Histones are conserved DNA-packaging proteins found across all domains of life. Here, we describe HLp from Leptospira perolatii and show by crystallographic and biophysical analyses that, unlike HBb, it forms stable tetramers and binds DNA nonspecifically, wrapping ~60 bp of DNA around its core. The HLp monomer exhibits the characteristic histone fold, comprising three α-helices (α1, α2, and α3) connected by two loops (l1 and l2). Molecular dynamics simulations, DNA-binding assays, and heterologous expression in Escherichia coli, where HLp reorganizes the nucleoid, support a role in bacterial chromatin organization.

To gain structural insight into the interaction between HLp and DNA, we co-crystallized HLp and the 30-bp-GC40 fragment. Diffraction data were collected for two different crystal forms, HLp-DNA_1 and HLp-DNA_2, processed to resolutions of 2.10 Å and 1.90 Å, respectively. Both structures were solved by molecular replacement using the DNA-free HLp structure as the search model. In HLp-DNA_2, the ASU comprises a single HLp monomer, which forms tetramers via crystallographic symmetry, and a 15-nt ssDNA segment of the apparently endless DNA. Although the overall crystal packing is similar to HLp-DNA_1, it exhibits a complementary DNA binding mode, with the dsDNA engaged along the HLp tetramerization interface. Therein, in both HLp dimers, the monomers bind to DNA via two sets of interactions. The first corresponds to the “β-bridge” motif in eukaryotic histones and involves T27 and G29 in loop l1, as well as T56 and T57 in loop l2, while the second set involves K17 and K21 from helix α1. The two DNA-bound crystal structures thereby reveal complementary, but overlapping DNA-binding interfaces distributed along the orbicular surface of the HLp tetramer, corresponding to the canonical interaction motifs of archaeal and eukaryotic histones. Crystal structures of HLp-DNA complexes reveal the HLp tetramer to be decorated with distinct DNA-binding interfaces along its perimeter, including motifs corresponding to the canonical “paired end of helices” and “β-bridge” motifs. While the two individual DNA-bound crystal structures might hint at a DNA-bridging mode, their structural superposition and the location of the individual DNA-binding motifs suggested a potential DNA-wrapping mode for HLp.

> GSMAQNAEKDTLIVASKVKAYIKSKGFMTSGDAVDGLNEKLYALIDDALKRTESNKRTTVRPTDF>[4x]GRKERERLEEKLEDANERIAELVKLEERQRIARDLEDTLGQKLSLIGLKSDLARKLIY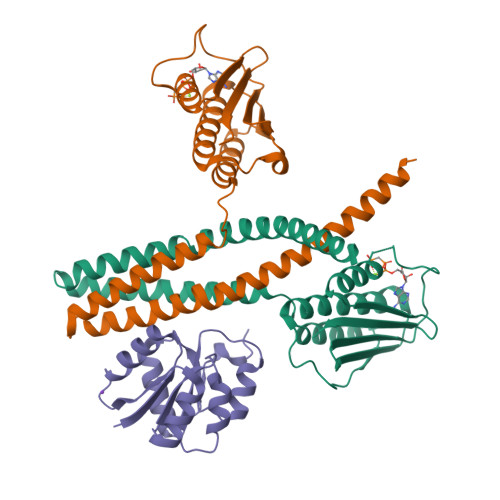KDPEQAARELKSVQQTARTSLNEVRKIVSSMKGIRLKDELINIKQILEAADIMFIYEEEKWPENISLLNENILSMCLKEAVTNVVKHSQAKTCRVDIQQLWKEVVITVSDDGTFKGEENSFSKGHGLLGMRERLEFANGSLHIDTENGTKLTMAIPNNSK;>[2x]GSGSMISIFIAEDQQMLLGALGSLLNLEDDMEVVGKGTTGQDAVDFVKKRQPDVCIMDIEMPGKTGLEAAEELKDTGCKIIILTTFARPGYFQRAIKAGVKGYLLKDSPSEELANAIRSVMNGKRIYAPELMEDLYSEA>MIVIFVDFDYFFAQVEEVLNPQYKGKPLVVCVYSGRTKTSGAVATANYEARKLGVKAGMPIIKAMQIAPSAIYVPMRKPIYEAFSNRIMNLLNKHADKIEVASIDEAYLDVTNKVEGNFENGIELARKIKQEILEKEKITVTVGVAPNKILAKIIADKSKPNGLGVIRPTEVQDFLNELDIDEIPGIGSVLARRLNELGIQKLRDILSKNYNELEKITGKAKALYLLKLAQDEYNEPIRTRVRKSIGRIVTMKRNS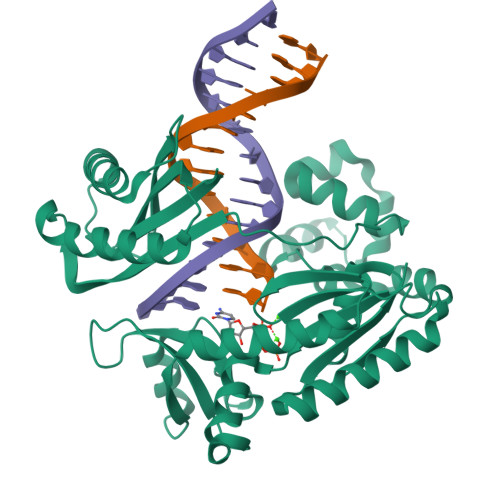RNLEEIKPYLFRAIEESYYKLDKRIPKAIHVVAVTEDLDIVSRGRTFPHGISKETAYSESVKLLQKILEEDERKIRRIGVRFSKFIEAIGLDKFFDTGGHHHHHH[2x]> MGELFLVGMGPGDLPGLTQRAREALEGAEVVIGYSTYVKLLEEMGLLAGKEVVRKGMTEEL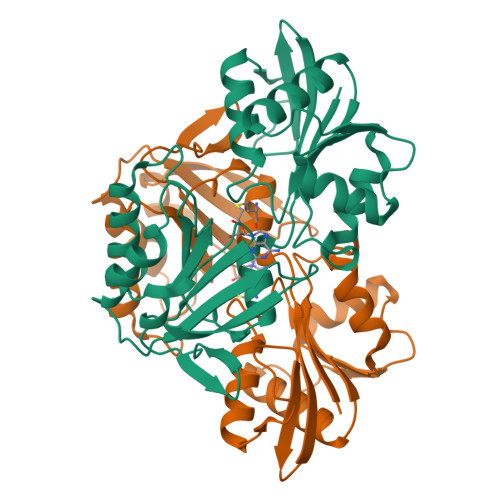DRAEEALERALSGQRVALVSGGDPGIYGMAAPVLELMEERGLKRVDGGVGLPGRFAGEEGEVFLAVIPGVTAANAVASLLGSPLAHDTCLISLSDLLTPWPLIERRLHAAGQGDFVVVLYNPQSKRRDWQLRKSAEILLEYRPKETPAALVKSAYRKRQEVALTTLEGLREAEAGMLTTVVIGNRQSRFYEGTFLTPRGYALKYDLDTKEALPGETPGLSLVSPEGASSGRRDA>GSAMGSSTSTSRATYMDRFNIPKNHVDLIWDKDGTKSHTRGNTTYRWTERKSNVGVYVGYSEMYDSSAQAYCQSSSAKIDTKTTVGAPYMAAGACPNYGKVIAFTKRDGSRSDMTRWKNEIHANVMPHSTTSCASRADPGAAEVAKSIEGFAMYAGYLTHCPYNVNVYRQDMVTDKEFDSTVCNFVTESNPLRFLDTTQRQSTQPYTEYAFHGKGGHKGYDYKGQTSHVGCPPYNPPHVTKGMKDSSWITGPFECSILSRCTTHCWPYKSGGNCFRSLPAMFDMSTGECRLLGYHTQDFRSSTCAELTTDDTNAFYCVRPMKTAASSNMVYVTSHTRPDHETKCPPREPLKNVRWGVVSKGKYCKPMNARASLSNATAEQCGQ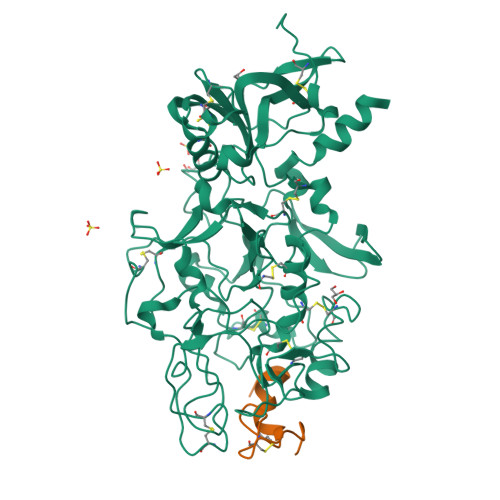RLFMLSSADGSSLSSQVRGYHWATFVATDCNMGESCAATARGKCFFYSTVPECLIHSPTTMAFTSLSAVDPSIAIDPDSIAVLPEDKCVSVDCGAHGTCDVATGKCVCEPGFTGERCDAAALVPR[2x];>[2x]GSASQIVQNQSSLAPELSGCPPMGICMDGTIGDPIAS> MSKTFAEIAEAFLEPEAVRIAKEAVEEYGDHERKIIQIGIHFQVCCMFCDEYLSTNGSDRFVLIEGRKRGTAVSLQNELCKSYDLEPLPFLCDIFDREEKQFVEIGITRKADDSYFQSKFGKLGNSCKIFVFSYDGRLDKNCEGPMEEQKLRIFSFLATAADFLRKENMFNEIFLPDNEETIIEMKKGKTFLELRDESVPLPFQTYEQMKDY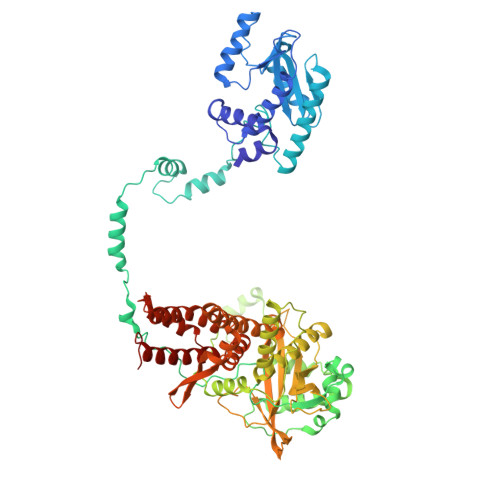CEKFKGNPRELASKVSQMQSNIKLPIKHYEQNKFRQIRLPKGPMAPYTHKFLMEEAWMFTKISDPERSRAGEILIDFFKKGNLSAIRPKDKPLQGKYPIHYKNLWNQIKAAIADRTMVINENDHSEFLGGIGRASKKIPEISLTQDVITTEGLKQSENKLPEPRSFPRWFNAEWMWAIKDSDLTGWVPMAEYPPADNELEDYAEHLNKTMEGVLQGTNCAREMGKCILTVGALMTECRLFPGKIKVVPIYARSKERKSMQEGLPVPSEMDCLFGICVKSKSHLNKDDGMYTIITFEFSIREPNLEKHQKYTVFEAGHTTVRMKKGESVIGREVPLYLYCRTTALSKIKNDWLSKARRCFITTMDTVETICLRESAKAEENLVEKTLNEKQMWIGKKNGELIAQPLREALRVQLVQQFYFCIYNDSQLEGFCNEQKKILMALEGDKKNKSSFGFNPEGLLEKIEECLINNPMCLFMAQRLNELVIEASKRGAKFFKTD>SDKIIHLTDDSFDTDVLKADGAILVDFWAEWCGPCKMIAPILDDIADEYQGKLTVAKLNIDQNPGTAPKYGIRGIP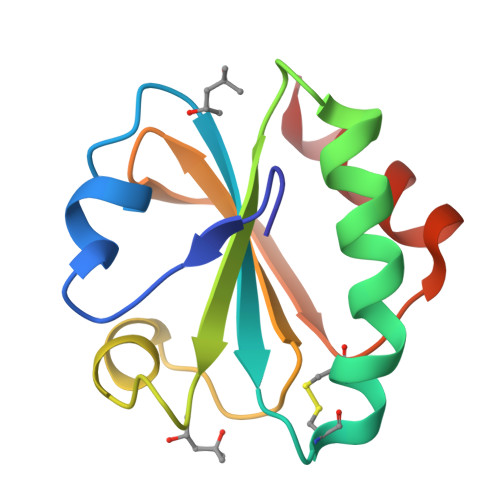TLLLFKNGEVAATKVGALSKGQLKEFLDANLA[2x]> MGSSHHHHHHSQDPNSMTTLTRQDLNFGQVVADVLCEFLEVAVHLILYVREVYPVGIFQKRKKYNVPVQMSCHPELNQYIQDTLHCVKPLLEKNDVEKVVVVILDKEHRPVEKFVFEITQPPLLSISSDSLLSHVEQ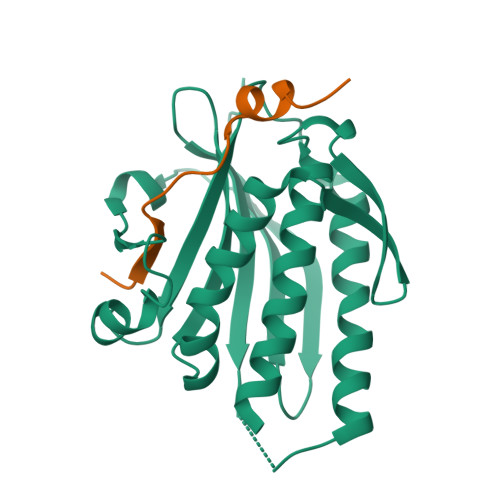LLAAFILKISVCDAVLDHNPPGCTFTVLVHTREAATRNMEKIQVIKDFPWILADEQDVHMHDPRLIPLKTMTSDILKMQLYVEERAHKGS;> MLTPTPDSSPRSTSSPSQSKNGSFTPRTANILKPLMSPPSREEIMATLLDHD>[4x]GSMDVVDPDIFNRDPRDHYDLLQRLGGGTYGEVFKARDKVSGDLVALKMVKMEPDDDVSTLQKEILILKTCRHANIVAYHGSYLWLQKLWICMEFCGAGSLQDIYQVTGSLSELQISYVCREVLQGLAYLHSQKKIHRDIKGANILINDAGEVRLADFGISAQIGAELARRLEFIGTPYWMAPEVAAVALKGGYNELCDIWSLGITAIELAELQPPLFDVHPLRVLFLMTKSGYQPPRLKEKGKWSAAF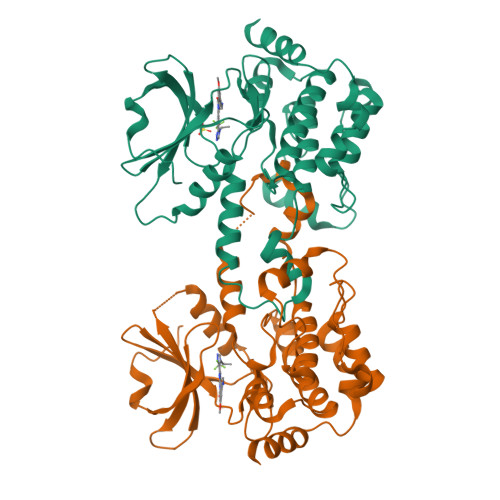HNFIKVTLTKSPKKRPSATKMLSHQLVSQPGLNRGLILDLLDKLKNPGKGPSIGDIEDEE>[3x]QSTEASPKRSDGTPFPWNKIRLPEYVIPVHYDLLIHANLTTLTFWGTTKVEITASQPTSTIILHSHHLQISRATLRKGAGERLSEEPLQVLEHPRQEQIALLAPEPLLVGLPYTVVIHYAGNLSETFHGF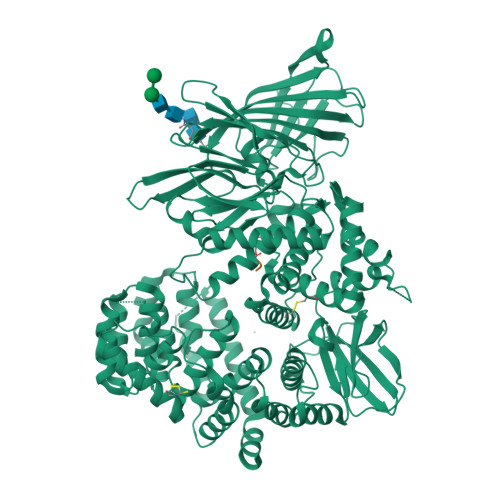YKSTYRTKEGELRILASTQFEPTAARMAFPCFDEPAFKASFSIKIRREPRHLAISNMPLVKSVTVAEGLIEDHFDVTVKMSTYLVAFIISDFESVSKITKSGVKVSVYAVPDKINQADYALDAAVTLLEFYEDYFSIPYPLPKQDLAAIPDFQSGAMENWGLTTYRESALLFDAEKSSASSKLDITMTVAHELAHQWFGNLVTMEWWNDLWLNEGFAKFMEFVSVSVTHPELKVGDYFFGKCFDAMEVDALNSSHPVSTPVENPAQIREMFDDVSYDKGACILNMLREYLSADAFKSGIVQYLQKHSYKNTKNEDLWDSMASICPTDGVKGMDGFCSRSQHSSSSSHWHQERVDVKTMMNTWTLQRGFPLITITVRGRNVHMKQEHYMKGSDGAPDTGYLWHVPLTFITSKSDMVHRFLLKTKTDVLILPEEVEWIKFNVGMNGYYIVHYEDDGWDSLTGLLKGTHTAVSSNDRASLINNAFQLVSIGKLSIEKALDLSLYLKHETEIMPVFQGLNELIPMYKLMEKRDMNEVETQFKAFLIRLLRDLIDKQTWTDEGSVSERMLRSELLLLACVHNYQPCVQRAEGYFRKWKESNGNLSLPVDVTLAVFAVGAQSTEGWDFLYSKYQFSLSSTEKSQIEFALCRTQNKEKLQWLLDESFKGDKIKTQEFPQILTLIGRNPVGYPLAWQFLRKNWNKLVQKFELGSSSIAHMVMGTTNQFSTRTRLEEVKGFFSSLKENGSQLRCVQQTIETIEENIGWMDKNFDKIRVWLQSEKLEHDPEADATGLERMLESRGPFEQKLISEEDLNMHTEHHHHHH;>XXTFPETLTY[3x]>[2x]GPGSEFELPLPEGWEEARDFDGKVY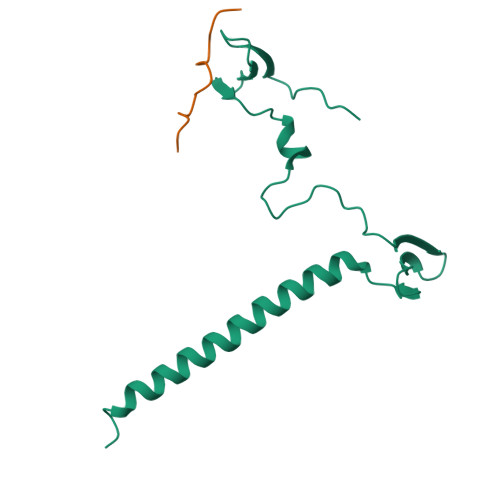YIDHRNRTTSWIDPRDRYTKPLTFADCISDELPLGWEEAYDPQVGDYFIDHNTKTTQIEDPRVQWRREQEHMLKDYLVVAQEALSAQKEIYQVKQQRLELAQQEYQQLH;>[2x]GPGSGRTEGQLMRYQHPPEYGAARPA> MSIQKSTNSSSLAEVIDRILDKGIVIDAFARVSVVGIEILTIEARVVIASVDTWLRYAEAVGLLRD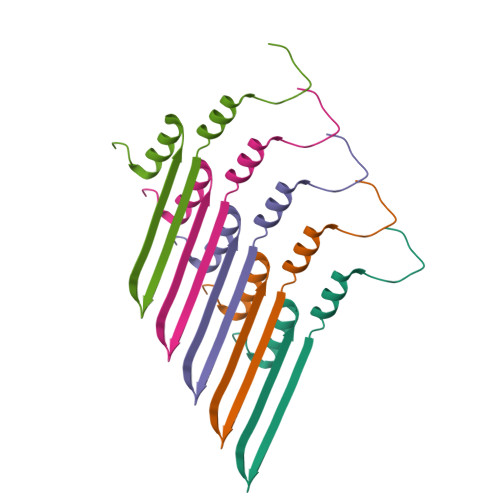DVEENGLPERSNSSEGQPRFSI> MDPRETAIGLVRYVTENAAKDFDGESIAAIIYRLRVVENYVSSDVDIICEAMRILIKKLVNLPPITFSPDVWMPIMTSITEGAIEPQWRIMMESIDISKFSSTSSNFVHMDSITASSTKCSEQITSICKGFALEFGLTRRLFSAIWNTDLEETARKMMNQEWDSVKIDSSPDSAKQAAGLIEKSIFDLFSEMKDHETFANELYYAALARILNNSRRLQENKKPAIQDSEDISFYESSLHIYDELIKKLWPHLSKKDPNVKKNTLIIFEKLISLSPTDVLVQRITEKFIDSCEWLKISGEEICTSMEPRLWKIVGSLVSRILDLKKTIPYEIVSYAIAVHITQEVTLASPEVSDCGPDSFDSTCDQPSNMKERFLRHMVDSYFQTRSSLLSIIQFLRTAKSSEEIVQFMRVFYPELVFGNETLITHAAIEMLRESASHHSIKADDFISIVLSVIDAPAIVRIIDVISCIKDEKVRKEAVEKTIIRMANDLEDEDQKREGYVNHLHENGSFWNDIAKYADASILDKAGKRFVEVSVDSMDIRSSVLATDIFLTILKLKLTSEAEREPESCVICNVSYSNIKIDLEKWNKMGNILVECNMVKRSKSEALPLFTIHQLENIDLPMRDLVYVVTQMKFLDTKEGMELHRKFYDGLPGVNVIFEKFMSKSHKIELCMKLLDEFAKIIAINEKSLIFSLDHENILDWLEEIGVLDSPQITEKLVDICFSIEVWDVLTLLQLDGPECHYWDLQMFGRFWKTSLMDLLDEKMMKKVNEKMGSILKEQYDKQSHVAKATREKRSNGKFPNRPKVADWEEQLLLMHNRIAGHLTKKKVEDFADESTQKFTWLLGVCSGQMSYKKEVAVDAEKILSRLYPDAEKRNEVLYHFGVSSILKGLDRPRGKLSLHILFMQIYLDLVQIDSKSWKIDDSVQKLSRRLGGFNEWLMIVDEEKREDDGGFRIYIVLNLSHYFWELLEGCKASQVVDAHAILKIRKFAEVLASILDKITFWPNPKLHAYYYIAQFLEPLETIFHFPEIAEQNRKVIESFFKQLFDKLLEQKYQEGLLQDTKLIIQKTDKYLSSSLNLFNEYNTQEPSKIYPVNEIFSLFCRYGSENVHLYCLKMIKKSLQTLASNILEHEHILKGEVCIETELQKRLVCDAVLLTEFFGYFSCIYAQVSENQPSEHDDVAKAFMLLDSDIHLKTKSRKRSTQNSVAVGSHRHQTAENMDLNFCTYKSTGRAYVTQHWYNCYTCNMMESEGVCSVCAINCHRGHDLAYSKKGSFFCDCGEKKCGAMQGIYHLPNSMYSLRGQLPEKNGDKTLPKIRNVFEHRFENLNSNCCDELKSALNDVQEEFKEVQDDLEQILEAVDFANQKALQVTEERLAVLESFNDMDDVIISEKEKFIEPLESGHFLPTRRDDLPVQELRVASSQHKIRELSDIIKLDDGTELLVLIPESIQTCLQLHYMDTRTNLIQGMHALRTETEQIPFNARSLHVSGNRLVVCGQYEFFALRFSPQGDVIDRAHIKLLENGASSSMNNNPVVRAKFCREIESDKRRRQLIAVATMQYIRIYDLTLHETNFVEEMVLPAGNVEDVEIINQEDGNVRILVLSSSGYLYEHNISVFNAENNSIFLTNVVNTPGMDMNGDGVSLHYSSTFNLLFVSLENGAFVAQLPEPTGNSTAPIYDWKHLNIKNPVDAWKETSGIIACLSTNCNHQVNYFHPTVGKILLQKTSVKRSIMTYFLMTSAKNQSVYSVLIYPNVPTCEIWETSWNNVHDLWIDDVPTERYAVEVVEQKSTQIPIDRDELVLLAEQCEQIRTVDWNCREIGMFYTHEELNNRLSSSDSLPITLIQQTHFKLSARITNFRQIVRMIRVEVEGNTGPEYLKIGTTRYSISSRGPKTFDLRLSREESLALDHRDITIEVIPRSNQNRVTLKSLRLLGCDRSAMDEIQPRYERQPILTNSNKLVYSILEFATLSGLEWAGNMAKKHLSRKLNHPAVCSVSTRAIVKCHPSVDEELFKIIDGAYLQEWKALIDWTESEGFGEMRLHHVEQLLDRMEAVRTRWPYFVKSLKREFGTVTSFVELMRNEMKRMPLHRCQMMAQAIVKIVFGLLSNGTNEAEQLIHVFLNIFTDQDTYHLANDMRSAVQETISRFENALKEEKKLMVEHENMDKESVLRIKNYGFSPFYGAPRIIAKTPESMLIAKIAETIPIDSEENFKWLEQLISMILEKLTRSNSTVTWQNLSDSPSYNLSRVLASCLAICDPVIIRNHFSRLIHIIKYDVEKIFPMSEKSYSNYSLLRSVELLLFVCLEKRGDESKENQEMLDSIVHDLQAVGIRNLCLKILEKVIPHWKDRGPSTFSRNSAESRKVWLPHVPLVSSSANPPNTSIMNWPSTSEDSYIIACTDLILLIPQHLQELDRRKSVPRDDQWIQKLCQLASLSSGCSAYRQCKKLLLAMCHNDENKYKIMRDKYKMQDLLQQLVKKYLDVSKEVGGHQQLTEIVDVLASITKLALIRPDMWRDVCSTHTTWLLRLACYTTDVVASQVVELLIVAVRDSSVGGQLSIQLADSIVEAENGEFIEKIIKRFLIGRDEQLRWTLHGMLRSVIQLASRQNQCILVKKLYNTIYPLAANLGVQGAQLVDLIATYAPRVFSSTELVAMTQSEISTIEKIRNTLNGDGYQGMYKLMSDLGLGWKSINFDRNPCLVCFTSKGSHDVVKMTSIKSDIRYSANTIIYKLISNYEVSKVTIKLTELKKSKSIKKVSLYYSAKSVESVDLKLHPELWRKCAMVTVAENETVINLSLAVPVVTSSLIVEFEEVVDHRGSSQLHCPRCTVPVRTHSGVCESCGENAFQCAKCRAINYVEKEPFLCQSCGFCKYAQISLFVVCRALPGAQHITCDAERGQCVQEITQLLIKMETTKTKLTGYRAACESLYLRNRPLPPYKLHVENNHTSEFFDANGTMNIEQLPFQSITMPMNNLAVAIRTLHSELCQQTQQLMYLHEELNRYDHASEVSVVFHKPQNISYYSTGQSCFGCLCNQLLHSVALLHSSCDDENALNLILSSDSLIEKLGVLAQTYETLREEVEELLVRLMFDRLDVTTKVEKLIHTGDINLSVMVKSLMYAADPTWQQKLKLLIRLAMDKRDENCCLQALMVLSKYLEATKSVTLDERKKIKLTPNKNITKWLTTDEEWKDCFSVASTSTAPTKSLPSNPYQWITDCLFSQWMSVRSAANQLLVNLSRQQFHEPVALLILCENMSKLSDVPSSVCDQFMCSAHTIIDSSVNTKARLFVQQFHVYLIKRIHEECAKLHEQSVNLLSDNMFGERLRCFVELLSLLLSGSNVENVLLKAGADDLLIFLLHSTIFLKRIMTRRTRATDSSRIALEKLLKRVSCRDGTKLMSVCVESLKLVKDTSTLGIIVGVMMEIMDPQQETEESFLIQIEKDIAQEDFLQGRMTHNPYNSSDPGMGPLMRDIKNKICRDTEMIALMEDDNGMELLVNGNIISLSLSVRDVYDRLWKRSNNGSPMLIVYRMRGLMGDAVETFIENFGVADNSEADDEEDEQLVRMTHCLMECGGIDKLMDLLTTNVDSSSGRFLLCYLRKIFERIVKIPIGRKILVQRRMVERMMSVIRTCCADPTNESKVLIGMELYKVVEFVVSDKHVQDILGGIREDDAMWWFDLFEKRGNEEGSVTELHRKTAQILDQMTMSIGNIVLGNDASEGVLVKMYEKVLKWEQIDSGAPPSGATDHQNRSRITKKDQIMLMTEQLATITSNIISSAHGIRLKQKILDSGVISSTCNYLTKDLPNLYQPTESPEWKVFLARPSLKLILTLLAGLARGHQASQKEIAKTTLKLMHRLEQVASDNSIGTLAENVIEALNEDEEVRNQIKLVRDETEKKKKQMAMLNREKQLTKMRMKVGTGGQIKVSSRTLHNEPSIDDSDSLPCCICRESVISGDKSAGVYAFAAIDPDSGKTSTVSMMVMVHFNCHKDAIRGGGGRAADEWTRSKLHNAGAKCNVITPISMGVVIGDAWIDALHRFENDVGRVSGLAHGVVNRNFVFVDICNLIDRFIYKRSFSNQSEGGGRESNMQYLAILHLLGITLPADAELEISAPNHRLIAFLFTELTADSWNDQRNDVLRAGINDAQTNGAPATWDGFKPTLMTWAFVDAYFNKVIKITGEDRLEWLREHLVETINKTRGFVDDFDSNILPCEDVAEFCDVTGAPIDDVNLFLAGGPPQGSLEVLFQGPAEAAAKEAAAKEAAAKEAAAKALEAEAAAKEAAAKEAAAKEAAAKAHHHHHHHHHH

Among the >600 human ubiquitin ligases, UBR4 plays a particularly important PQC role, being an essential and conserved E3/E4 ligase found across eukaryotes. Aside from teaming up with various ubiquitin ligases, UBR4 activity is linked to two specific cofactors: calcium-binding protein calmodulin (CALM1) and KCMF1 (13, 16, 17, 20, 21). Our data show that the evolutionarily conserved UBR4 complex forms a megadalton E4 arena, in which inward-facing ZZ-DZB domains of KCMF1 act not as E3 ligases but as substrate receptors. The architecture of the E4 megacomplex is conserved across eukaryotes, but species-specific adaptations allow UBR4 to perform its precisely tuned quality-control function in diverse cellular environments.

To explore structural differences, we determined the cryo-EM structure of CeUBR4. Although the nematode E4 complex preserves the ring shape of the human enzyme, it displays notable adaptations, particularly in the dimerization interfaces that result in different topologies of the ring-shaped arena. Proteomic analysis of purified CeUBR4 pointed to a distinct substrate preference, with mitochondrial medium-chain acyl-CoA dehydrogenase (ACADM) showing stronger enrichment compared to SSBP1, which is preferred by the human UBR4 complex. In line with this finding, we observed well-defined extra density in the central arena of CeUBR4, closely resembling the elongated shape of an orphaned subunit from the tetrameric ACADM complex. The functional importance of the ring architecture is emphasized by its conserved shape and dimension in CeUBR4, despite pronounced differences in its helical scaffold and dimerization interfaces.> MVLIDMSVDLSTQVVDHYENPRNVGSLDKTSKNVGTGLVGAPACGDVMKLQIQVDEKGKIVDARFKTFGCGSAIASS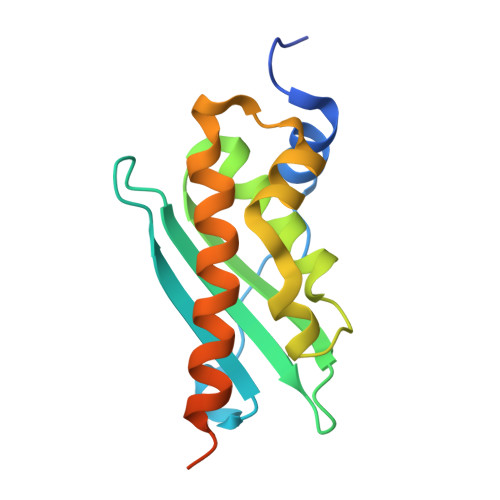SLATEWVKGKTVEEALTIKNTDIAKELCLPPVKLHCSILAEDAIKAALADYKLKQEPKKGEAEKKELHHHHHH> GAMGSMSKSLKKLVEESREKNQPEVDMSDRGISNMLDVNGLFTLSHITQLVLSHNKLTMVPPNIAELKNLEVLNFFNNQIEELPTQISSLQKLKHLNLGMNRLNTLPRGFGSLPALEVLDLTYNNLSENSLPGNFFYLTTLRALYLSDNDFEILPPDIGKLTKLQILSLRDNDLISLPKEIGELTQLKELHIQG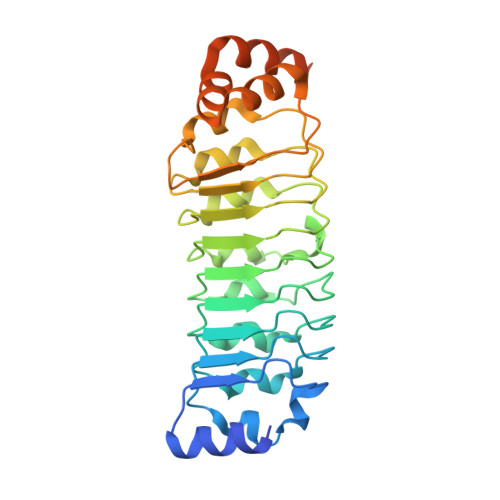NRLTVLPPELGNLDLTGQKQVFKAENNPWVTPIADQFQLGVSHVFEYIRSETYKYLYGRHMQANPEPPKKNNDKSKKISRKPLAAKNR> TKYKWTRTKVDIAEGPGTMNMANVLSTTGAQSVALVGERAFYDPRTAGSKSRFDDMIKIAQLFSVMSDNTTPSSSSGIDKYGYFDWAATVAPQNMVHRNVVTLDQFPNLNLFMNTYSYFRGSL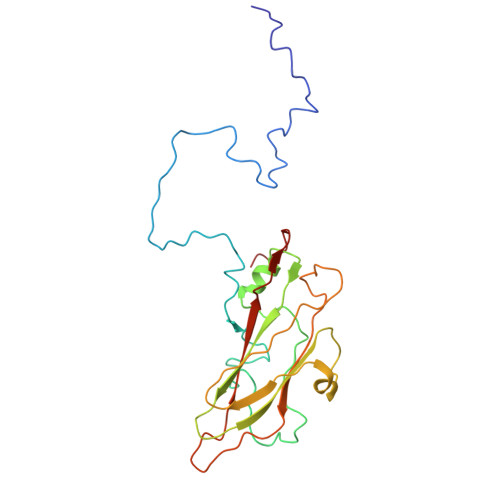IIRLSIYASTFNRGRLRMGFFPNCTHDTQLELDNAIYTICDIGSDNSFELTIPYSFSTWMRKTHGHQLGLFQVEVLNRLTYNSSSPNKVHCIVQGRLGDDAKFFCPTGSLVSFQ> MWMPPRPEEVARKLRRLGFVERMAKGGHRLYTHPD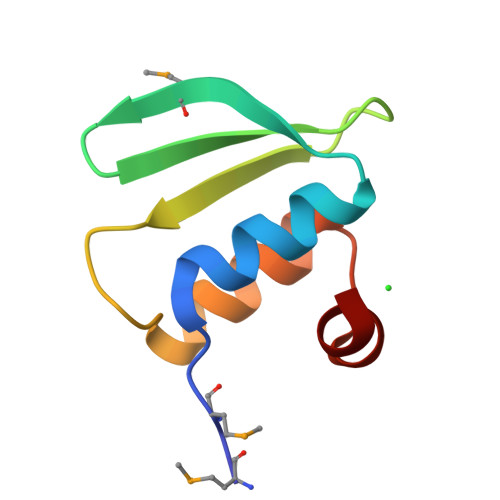GRIVVVPFHSGELPKGTFKRILRDAGLTEEEFHNL>MQKQAELYRGKAKTVYSTENPDLLVLEFRNDTSAGDGARIEQFDRKGMVNNKFNYFIMSKLAEAGIPTQMERLLSDTECLVKKLDMVPVECVVRNRAAGSLVKRLGIEEGIELNPPLFDLFLKNDAMHDPMVNESYCETFGWVSKENLARMKELTYKANDVLKKLFDDAGLILVDFK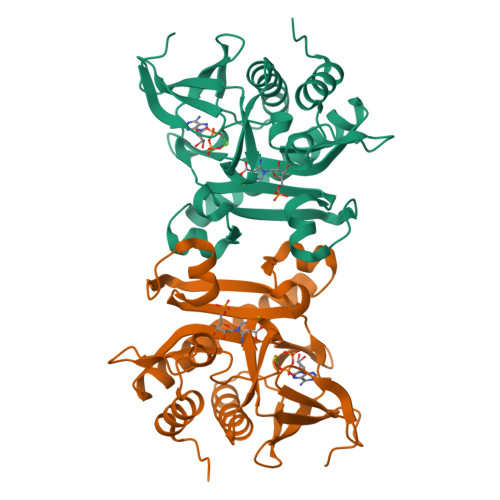LEFGLYKGEVVLGDEFSPDGSRLWDKETLEKMDKDRFRQSLGGLIEAYEAVARRLGVQLD[2x]> SALRLQMLGTGGAFAKKYFNNNALLYAGDFTLLIDCGITAPLALHTIGKSVEEIDAVLITHIHGDHVGGLEELAFRRKFGSGRKPILYIAENLVEPLWENTLKGGLSQDGVIHSLNDVFDVRLLKESEPAQLAPELKVELIRTPHIPGKPSYSLYINDEIFYSADMTFEPELLMRLVRERGCRRIFHEVQLTGKGEVHTTLQELLSLPTEIQSQILLKHYSDDMESFRGATGNMDFLRQHEVYTL

The cyclic oligonucleotide-based antiphage signalling system (CBASS) and the pyrimidine cyclase system for antiphage resistance (Pycsar) are antiphage defence systems in diverse bacteria that use cyclic nucleotide signals to induce cell death and prevent viral propagation. Here we show that phages encode anti-CBASS (Acb) and anti-Pycsar (Apyc) proteins that counteract defence by specifically degrading cyclic nucleotide signals that activate host immunity. Using a biochemical screen of 57 phages in Escherichia coli and Bacillus subtilis, we discover Acb1 from phage T4 and Apyc1 from phage SBSphiJ as founding members of distinct families of immune evasion proteins. We confirmed the critical role for Apyc1 metal-coordinating residues and identified E74 and Y112 from the opposing protomer as further catalytic residues required for cCMP hydrolysis and release of the reaction product 5′-CMP. Together, these findings demonstrate that Acb1 and Apyc1 constitute separate families of immune evasion proteins and explain the distinct reaction mechanisms that degrade CBASS or Pycsar cyclic nucleotide signals.

To compare mechanisms of anti-CBASS and anti-Pycsar evasion, we determined the crystal structure of Apyc1 from the phage Bsp38 (2.7 Å) as well as structures of Paenibacillus Apyc1 proteins (1.5 Å and 1.8 Å). In a structure of Paenibacillus Apyc1 co-crystallized in the presence of nonhydrolysable cAMP, we observed strong electron density near the Zn2+ ions and more diffuse density in the nucleobase pocket, consistent with specific coordination of the phosphate and ribose backbone of cyclic mononucleotides and weaker nucleobase specificity within the enzyme active site. Structures of Apyc1 reveal a metal-dependent cyclic NMP phosphodiesterase that uses relaxed specificity to target Pycsar cyclic pyrimidine mononucleotide signals. We identified 107 proteins related to Apyc1 present in phage genomes and also found many closely related bacterial proteins encoded in diverse bacterial orders. Similar to SBSphiJ Apyc1, closely related phage and bacterial Apyc1-like proteins cleaved cyclic mononucleotides with broad specificity. Structural comparison of Apyc1 and B. subtilis YhfI also reveals that Apyc1 enzymes contain an extended loop that reaches into the nucleotide-binding pocket, potentially enabling stable binding of smaller cyclic pyrimidine substrates.Thymidylate synthase (TS, EC 2.1.1.45) is a ubiquitous enzyme that catalyses the reductive methylation of 2’-deoxyuridine-5’-monophosphate (dUMP) to 2’-deoxythymidyne-5’-monophosphate (dTMP) using N5,N10-methylenetetrahydrofolate (mTHF) as cofactor. In human cells, TS provides the only synthetic source of dTMP necessary for DNA biosynthesis. hTS is an obligate homodimer with residues from both subunits that contribute to create the substrate binding site. Former structural analysis on hTS has revealed that the enzyme homodimers can switch between the active and the inactive conformation, primarily differing in the orientation of the catalytic loop (residues 181–197).

The replacement of Arg175 with a cysteine results in the complete loss of enzyme activity, proving that Arg175 is fundamental to anchor the substrate inside the catalytic cavity. The structure of the HT-hTS R175C was solved to 2.25 Å resolution, showing the constitutive dimeric quaternary structure of the enzyme. Within each enzyme homodimer, both subunits adopt the active conformation, showing the catalytic Cys195 exposed inside the active site cavity. In all subunits, Cys195 results oxidized to S-oxy-cysteine (CSX195). Indeed, an extra-electron density, whose shape is highly compatible with a folate-like molecule, is observed in only one catalytic cavity of each dimer. The refinement demonstrated that the ligand is a tetrahydrofolate (THF) derivative since the pyrazine ring of the folate pteridine moiety was in a bent conformation peculiar of the cofactor reduced form. 5-FTHF is stabilized into the cofactor binding site of HT-hTS R175C by a tight network of H-bonds and van der Waals interactions in analogous pose to that assumed in EfTS. Nonetheless, HT-hTS R175C displays the active conformation despite the high-salt condition (precipitant solution including 25 % saturated ammonium sulfate, corresponding to a concentration of ~ 1 M) applied to crystallize the protein. Even though the variant is able to accommodate a sulfate anion in this site, its catalytic inefficiency indicates that dUMP binding is impaired, strongly suggesting that Arg175 is pivotal to anchor the substrate.

>[4x]MRGSHHHHHHGSMPVAGSELPRRPLPPAAQERDAEPRPPHGELQYLGQIQHILRCGVRKDDRTGTGTLSVFGMQARYSLRDEFPLLTTKRVFWKGVLEELLWFIKGSTNAKELSSKGVKIWDANGSRDFLDSLGFSTREEGDLGPVYGFQWRHFGAEYRDMESDYSGQGVDQLQRVIDTIKTNPDDCRIIMCAWNPRDLPLMALPPCHALCQFYVVNSELSCQLYQRSGDMGLGVPFNIASYALLTYMIAHITGLKPGDFIHTLGDAHIYLNHIEPLKIQLQREPRPFPKLRILRKVEKIDDFKAEDFQIEGYNPHPTIKMEMAV>[2x]GSGFTSKDTYLSHFNPRDYLEKYYKFGSRHSAESQILKHLLKNLFKIFCLDGVKGDLLIDIGSGPTIYQLLSACESFKEIVVTDYSDQNLQELEKWLKKEPAAFDWSPVVTYVCDLEGNRVKGPEKEEKLRQAVKQVLKCDVTQSQPLGAVPLPPADCVLSTLCLDAACPDLPTYC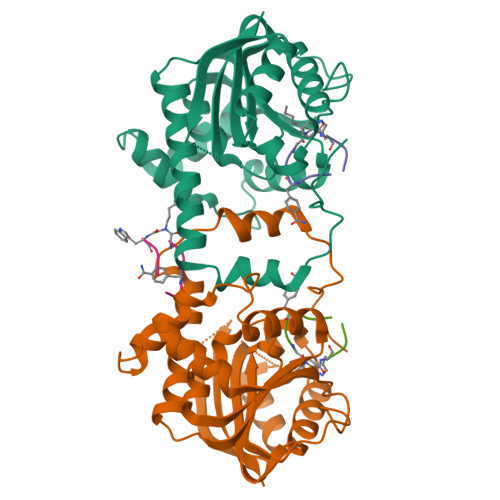RALRNLGSLLKPGGFLVIMDALKSSYYMIGEQKFSSLPLGREAVEAAVKEAGYTIEWFEVISQSYSSTMANNEGLFSLVARKL;>[3x]GFFRGXWPCG>[2x]MVLYFIGLGLYDERDITVKGLEIAKYCDYVFAEFYTSLMAGTTLGR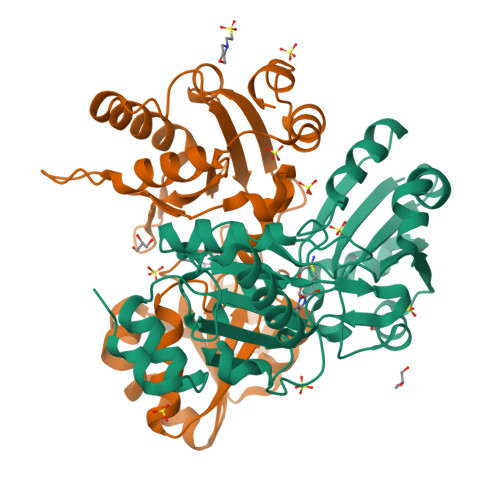IQKLIGKEIRVLSREDVELNFENIVLPLAKENDVAFLTPGDPLVATTHAELRIRAKRAGVESYVIHAPSIYSAVGITGLHIYKFGKSATVAYPEGNWFPTSYYDVIKENAERGLHTLLFLDIKAEKRMYMTANEAMELLLKVEDMKKGGVFTDDTLVVVLARAGSLNPTIRAGYVKDLIREDFGDPPHILIVPGKLHIVEAEYLVEIAGAPREILRVNV> TEETSITNFYSRAGLVGVVNMPVQGTSNTKGFAKWGIDIMGFVQMRRKLELMTYMRFSAEFTFVASTPEGETTNLILQYMYAPPGAPLPTRRDSYEWQTSTNPSIISKMADPPAQVSVPFLSPASAYQWFYDGYPTFGKHPIDQDFQYGMCPNNMMGTFCVRMIGGGKPTQSVTIRIYMRLKHIRAWVPRPLRSQNYTMRNYPN;> SPTAEACGYSDRVAQLTVGNSTI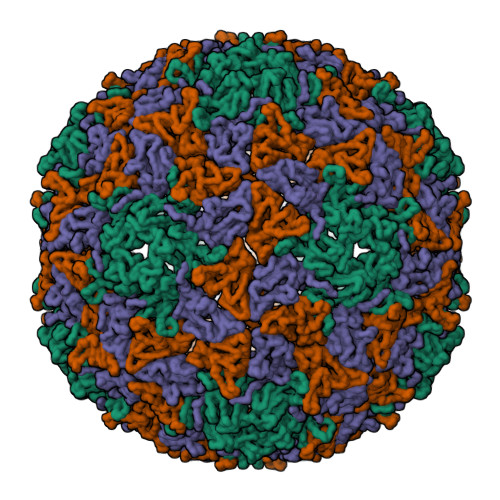TTQEAANVIVAYGEWPQYCPDTDATAVDKPTRPDVSVNRFYTLDTKDWSSSSKGWYWKFPDILAETGVFGQNAQFHFLYRSGFCIHVQCNASKFHQGALLVAVLPEYVTGTVSGNTGHENTHPPYAATQPGATGFELTNPYILDAGIPLSQLLVCPHQWINLRTNNCATIVVPYINSVPFDSALNHCNFGLVVIPVSPLGFLQGATPTIPITITVAPMNSEFSGLRQAVTQ;> RNLLELCQIDTIMEVNNLTTNEATPMERLRIPVQVQTQSGELCAAFKADPGLDGPWQSTMVGQLCRYYTQWSGSLKITFMFTGSFMATGKMLIAYTPPGGSLPANRMQAMLGTHVIWDFGLQSSVTLVVPWISNTHYRSQATGSFFDYYATGIVSLWYQTNFVVPIGAPTTAYIVVLGSAQKNFTMRLCRDTSELTQAAEYQ>MVKTQRVVITPGEPAGIGPDLVVQLAQREWPVELVVCADATLLTNRAAMLGLPLTLRPYSPNSPAQPQTAGTLTLLPVALRAPV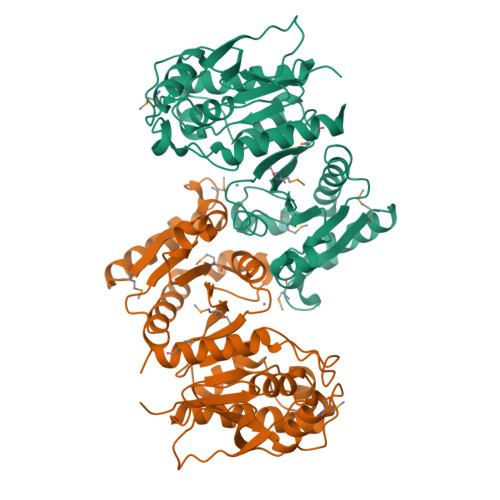TAGQLAVENGHYVVETLARACDGCLNGEFAALITGPVHKGVINDAGIPFTGHTEFFEERSQAKKVVMMLATEELRVALATTHLPLRDIADAITPALLHEVIAILHHDLRTKFGIAEPRILVCGLNPHAGEGGHMGTEEIDTIIPVLNELRAQGMKLNGPLPADTLFQPKYLDNADAVLAMYHDQGLPVLKYQGFGRGVNITLGLPFIRTSVDHGTALELAGRGKADVGSFITALNLAIKMIVNTQ[4x]>XIEELLRKILEDEARHVAEL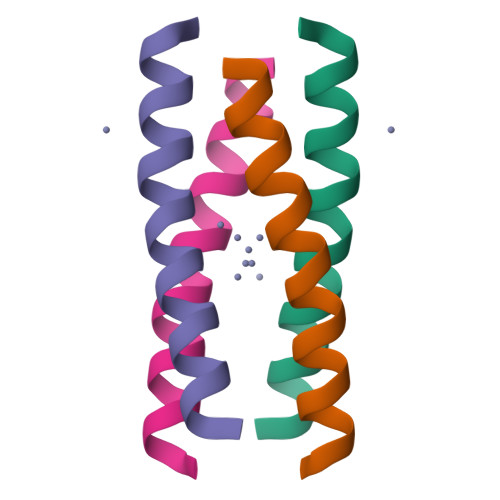EDIEKWLX[4x]>[4x]AAPILFWHRRDLRLSDNIGLAAARAQSAQLIGLFCLDPQILQSADMAPARVAYLQGCLQELQQRYQQAGSRLLLLQGDPQHLIPQLAQQLQAEAVYWNQDI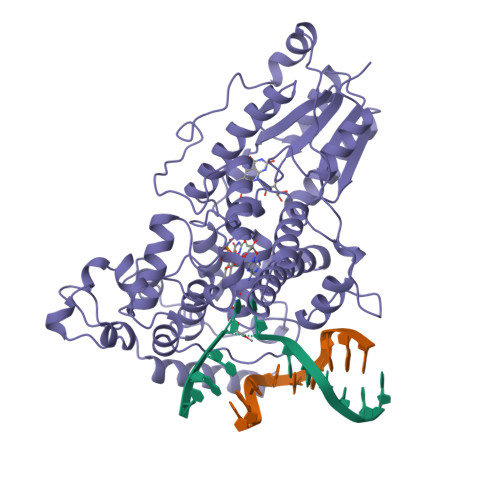EPYGRDRDGQVAAALKTAGIRAVQLWDQLLHSPDQILSGSGNPYSVYGPFWKNWQAQPKPTPVATPTELVDLSPEQLTAIAPLLLSELPTLKQLGFDWDGGFPVEPGETAAIARLQEFCDRAIADYDPQRNFPAEAGTSGLSPALKFGAIGIRQAWQAASAAHALSRSDEARNSIRVWQQELAWREFYQHALYHFPSLADGPYRSLWQQFPWENREALFTAWTQAQTGYPIVDAAMRQLTETGWMHNRCRMIVASFLTKDLIIDWRRGEQFFMQHLVDGDLAANNGGWQWSASSGMDPKPLRIFNPASQAKKFDATATYIKRWLPELRHVHPKDLISGEITPIERRGYPAPIVNHNLRQKQFKALYNQLKAAI>MTKKRIAVIGAGASGLTSIKCCLEEGLEPVCFERTDDIGGLWRFQENPEEGRASIYKSVIINTSKEMMCFSDYPIPDHYPNFMHNSQVLEYFRMYAKEFDLLKYIQFKTTVCSVKKQPDFSTSGQWEVVTECEGKKEVDVFDGVMVCTGHHTNAHLPLESFPGIEKFKGQYFHSRDYKNPEGFTGKRVIIIGIGNSGGDLAVEISHTAKQVFLSTRRGAWILNRVGDHGYPFDVLFSSRFTYFLSKICGQ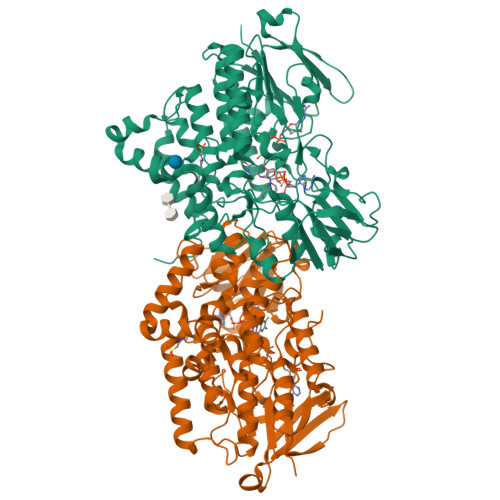SLSNTFLEKKMNQRFDHEMFGLKPKHRALSQHPTVNDDLPNRIISGLVKVKGNVKEFTETAAIFEDGSREDDIDAVIFATGYSFAFPFLEDSVKVVKNKVSLYKKVFPPNLEKPTLAIIGLIQPLGAIMPISELQGRWATQVFKGLKTLPSQSEMMAEISKAQEEMAKRYVDSQRHTIQGDYIDTMEEIADLVGVRPNLLSLAFTDPKLALKLFFGPCTPVQYRLQGPGKWDGARKTILTTEDRIRKPLMTRVIEKSNSMTSTMTMGRFMLAVVFFAIIMAYF[2x]>EHGPVTFVPDTPIESRARLSLPKQLVLRQSIVGAEVGVWTGETIPVRTCFGPLIGQQSHSMEVAEWTDKAVNHIWKIYHNGVLEFCIITTDENECNWMMFVRKARNREEQNLVAYPHDGKIFFCTSQDIPPENELLFYYSRDYAQQIGVP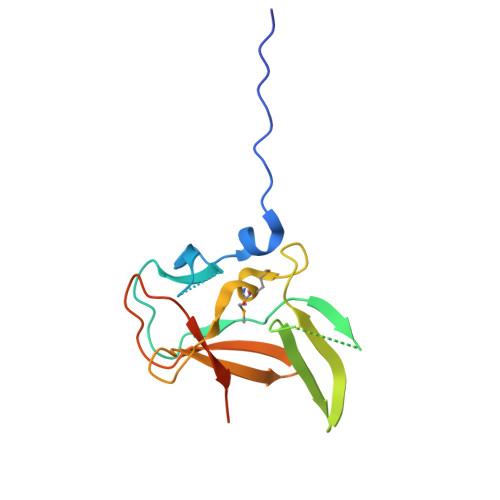E[2x]>GGEPAWDSPLRRVLAELNRIPSSRRRAARLFEWLIAPMPPDHFYRRLWEREAVLVRRQDHTYYQGLFSTADLDSMLRNEEVQFGQHLDAARYINGRRETLNPPGRALPAAAWSLYQAGCSLRLLCPQAFSTTVWQFLAVLQEQFGSMAGSNVYLTPPNSQGFAPHYDDIEAFVLQLEGRKLWRVYRPRVPTEELALTSSPNFSQDDLGEPVLQTVLEPGDLLYFPRGFIHQAECQDGVHSLHLTLSTYQRNTWGDFLEAILPLAVQAAMEENVEFRRGLPR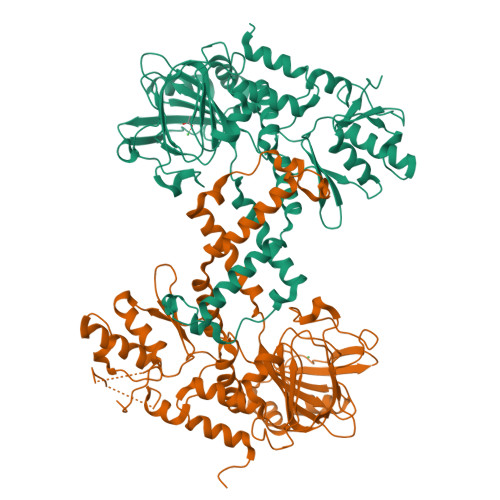DFMDYMGAQHSDSKDPRRTAFMEKVRVLVARLGHFAPVDAVADQRAKDFIHDSLPPVLTDRERALSVYGGGGQLTTETEVHMLQDGIARLVGEGGHLFLYYTVENSRVYHLEEPKCLEIYPQQADAMELLLGSYPEFVRVGDLPCDSVEDQLSLATTLYDKGLLLTKMPLALN[2x]N-methyl-1-phenylmethanamine | C8 H11 N | 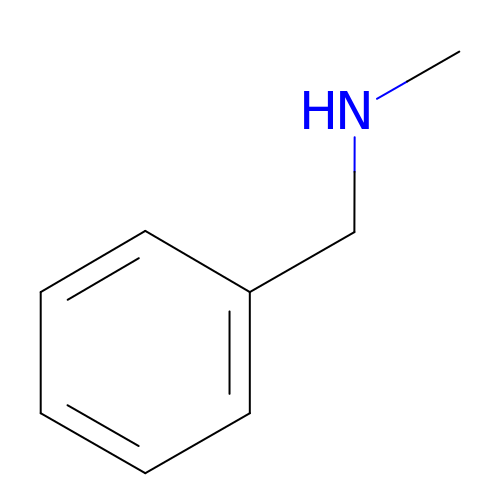RIWRFSMVIUAEBX-UHFFFAOYSA-N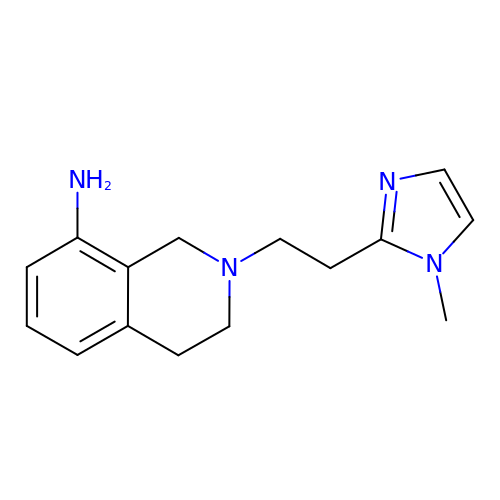2-[2-(1-methyl-1H-imidazol-2-yl)ethyl]-1,2,3,4-tetrahydroisoquinolin-8-amine | C15 H20 N4 | JGJLPCQCNSYHGF-UHFFFAOYSA-N>[4x]MGLRSVFVSGFPRDVDSAQLSEYFLAFGPVASVVMDKDKGVFAIVEMGDVGAREAVLSQSQHSLGGHRLRVRPR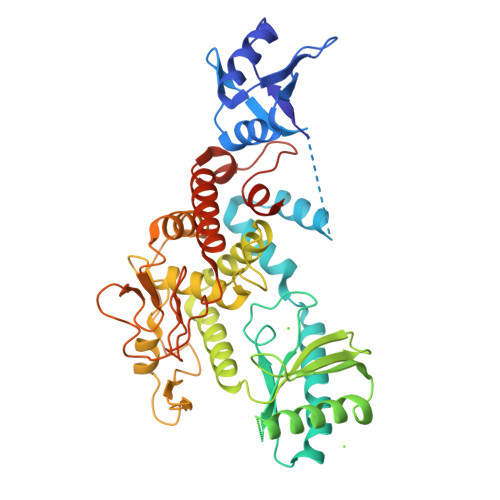EQKEFQSPASKSPKGAAPDSHQLAKALAEAADVGAQMIKLVGLRELSEAERQLRSLVVALMQEVFTEFFPGCVVHPFGSSINSFDVHGCDLDLFLDLGDLEEPQPVPKLPPASPLLEDREEGDLGKASELAETPKEEKAEGAAMLELVGSILRGCVPGVYRVQTVPSARRPVVKFAHRPSGLHGDVSLSNRLALHNSRFLSLASELDGRVRPLVYTLRAWAQGRGLSGSGPLLSNYALTLLVIYFLQTRDPPVLPTVSQLTQKAGEGEQVEVDGWDCSFPRDASRLEPSINVEPLSSLLAQFFSAVSSWDLRGSLLSLREGQALPVAGGLPSNLWEGLRLGPLNLQDPFDLSHNVAANVTSRVAGRLQNCCRAAANYARSLQYQRRSSRGRDWGLLPLLQPSSLEHHHHHH>[2x]ASAWPEEKNYHQPAILNSSALRQIAEGTSISEMWQNDLQPLLIERYPGSPGSYAARQHIMQRIQRLQADWVLEIDTFLSQTPYGYRSFSNIISTLNPTAKRHLVLACHYDSKYFSHWNNRVFVGATDSAVPCAMMLELARALDKKLLSLKT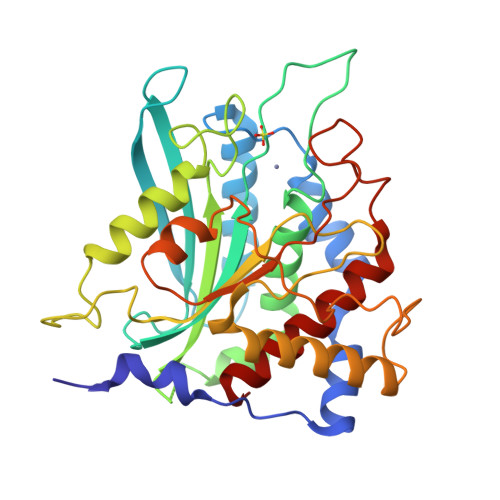VSDSKPDLSLQLIFFDGEEAFLHFSPQDSLYGSRHLAAKMASTPHPPGARGTSQLHGMDLLVLLDLIGAPNPTFPNFFPNSARWFERLQAIEHELHELGLLKDHSLEGRYFQNYSYGGVIQDDHIPFLRRGVPVLHLIPSPFPEVWHTMDDNEENLDESTIDNLNKILQVFVLEYLHL>[4x]AAAVRSVKGLVAVITGGASGLG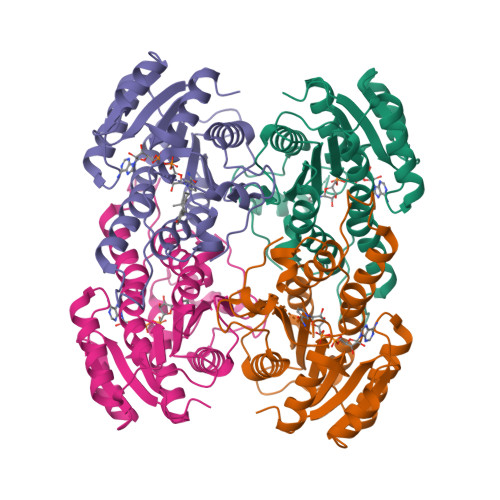LSTAKRLVGQGATAVLLDVPNSEGETEAKKLGGNCIFAPANVTSEKEVQAALTLAKEKFGRIDVAVNCAGIAVAIKTYHEKKNQVHTLEDFQRVINVNLIGTFNVIRLVAGVMGQNEPDQGGQRGVIINTASVAAFEGQVGQAAYSASKGGIVGMTLPIARDLAPIGIRVVTIAPGLFATPLLTTLPDKVRNFLASQVPFPSRLGDPAEYAHLVQMVIENPFLNGEVIRLDGAIRMQP> PTGLAADIRWTAYGVPHIRAKDERGLGYGIGYAYARDNACLLAEEIVTARGERARYFGSEGKSSAELDNLPSDIFYAWLNQPEALQAFWQAQTPAVRQLLEGYAAGFNRFLREADGKTTSCLGQPWLRAIATDDLLRLTRRLLVEGGVGQFADALVAAAPPGAEK;> SNAIAVGSERSADGKGMLLANPHFPWNGAMRFYQMHLTIPGRLDVMGASLPGLPVVNIGFSRHLAWTHTVDTSSHFTLYRLALDPKDPRRYLVDGRSLPLEEKSVAIEVRGADGKLSRVEHKVYQSIYGPLVVWPGKLDWNRSEAYALRDANLENTRVLQQWYSINQASDVADLRRRVEALQGIPWVNTLAADEQGNALYMNQSVVPYLKPELIPACAIPQLVAEGLPALQGQDSRCAWSRDPAAAQAGITPAAQLPVLLRRDFVQNSNDSAWLTNPASPLQGFSPLVSQEKPIGPRARYALSRLQGKQPLEAKTLEEMVTANHVFSADQVLPDLLRLCRDNQGEKSLARACAALAQWDRGANLDSGSGFVYFQRFMQRFAELDGAWKE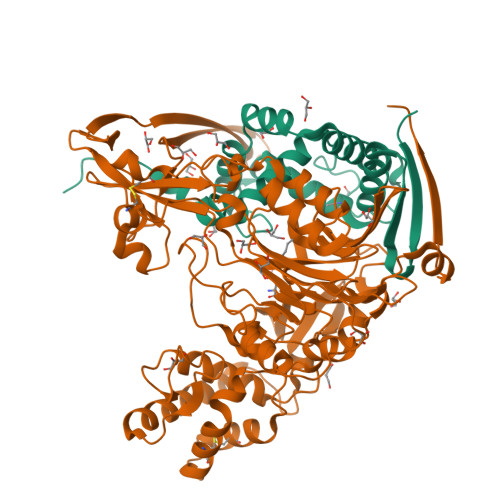PFDAQRPLDTPQGIALDRPQVATQVRQALADAAAEVEKSGIPDGARWGDLQVSTRGQERIAIPGGDGHFGVYNAIQSVRKGDHLEVVGGTSYIQLVTFPEEGPKARGLLAFSQSSDPRSPHYRDQTELFSRQQWQTLPFSDRQIDADPQLQRLSIREAA>SMEVARAARLAQIFKEICDGIISYKDSSRQALAAPLLNLPPKKKNADYYEKISDPLDLITIEKQILTGYYKTVEAFDADMLKVFRNAEKYYGRKSPVGRDVCRLRKAYYNARHEASAQIDEIVGET[2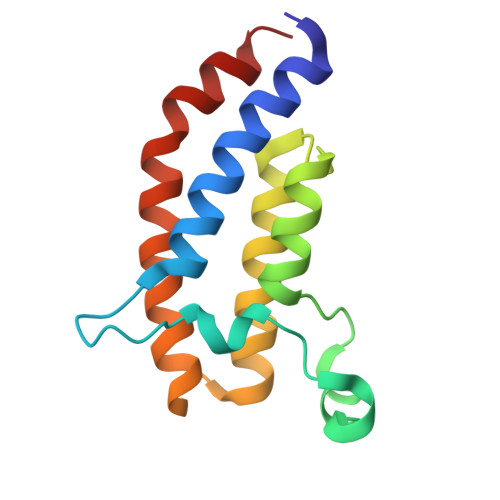x]> GSHMSTGDFLTKGIELVQKAIDLDTATQYEEAYTAYYNGLDYLMLALKYEKNPKSKDLIRAKFTEYLNRAEQLKKHLESEE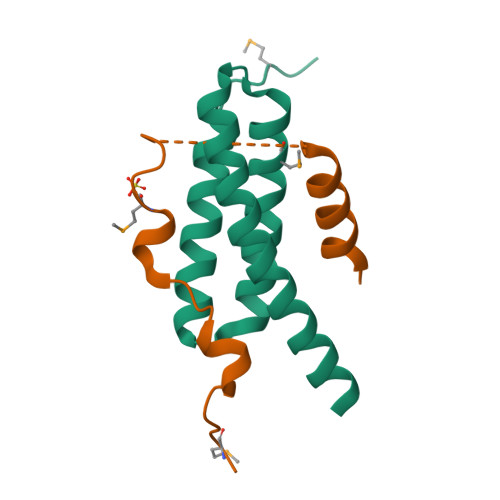ANAA;> GSHMLQSTPQNLVSNAPIAETAMGIAEPIGAGSEFHGNPDDDLQARLNTLKKQT1-[(1R,6R)-9-azabicyclo[4.2.1]non-2-en-2-yl]ethanone | C10 H15 N O | 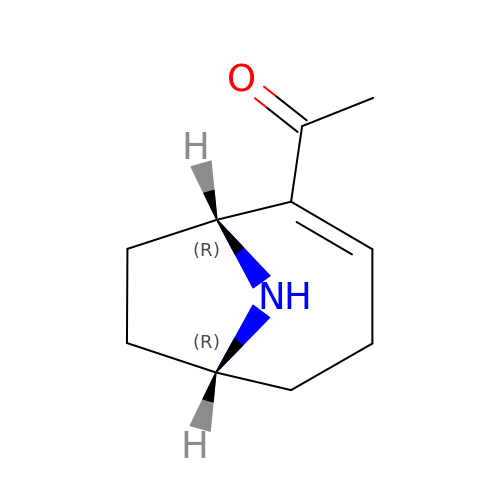SGNXVBOIDPPRJJ-PSASIEDQSA-N> AEEEI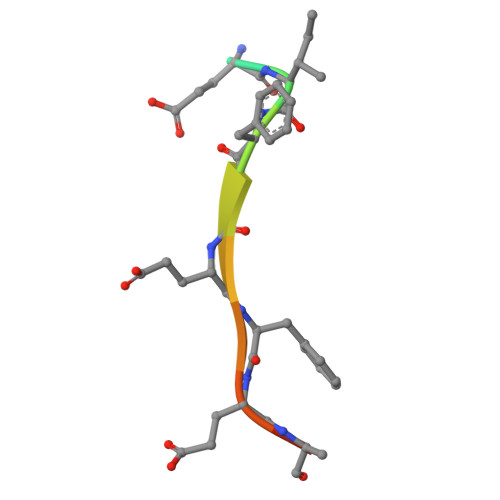FGEFEAKK(2~{R},4~{S},5~{R},6~{R})-5-acetamido-2-[4-[(2~{S})-3-[2-[(2~{S},3~{R},4~{R},5~{R},6~{R})-6-(hydroxymethyl)-3,4,5-tris(oxidanyl)oxan-2-yl]ethylamino]-3-oxidanylidene-2-(2-phenylethanoylamino)propyl]-1,2,3-triazol-1-yl]-4-oxidanyl-6-[(1~{R},2~{R})-1,2,3-tris(oxidanyl)propyl]oxane-2-carboxylic 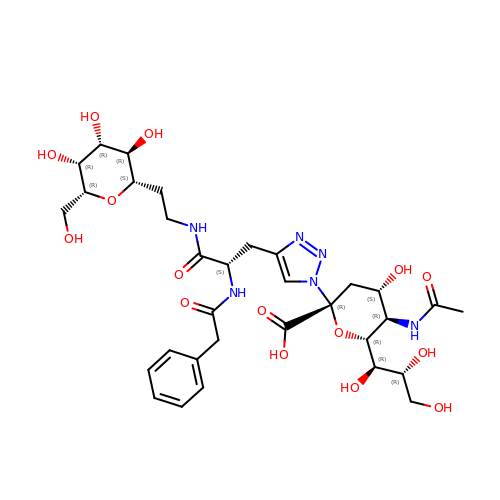acid | C32 H46 N6 O15 | VJJPXKHAIAQVCK-WZAWTCGUSA-N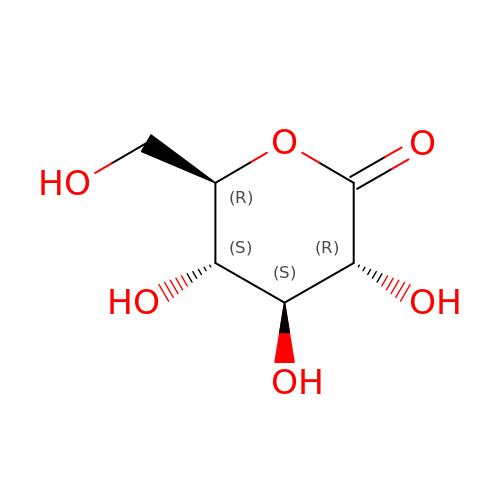D-glucono-1,5-lactone | C6 H10 O6 | PHOQVHQSTUBQQK-SQOUGZDYSA-N>[2x]APRKFFVGGNWKMNGDKKSLGELIHTLNGAKLSADTEVVCGAPSIYLDFARQKLDAKIGVAAQ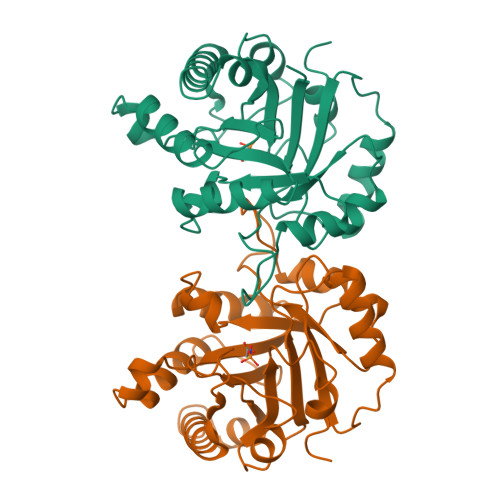NCYKVPKGAFTGEISPAMIKDIGAAWVILGHSERRHVFGESDELIGQKVAHALAEGLGVIACIGEKLDEREAGITEKVVFEQTKAIADNVKDWSKVVLAYEPVWAIGTGKTATPQQAQEVHEKLRGWLKTHVSDAVAQSTRIIYGGSVTGGNCKELASQHDVDGFLVGGASLKPEFVDIINAKH> MTLKGMSYVMCTGSFKLEKE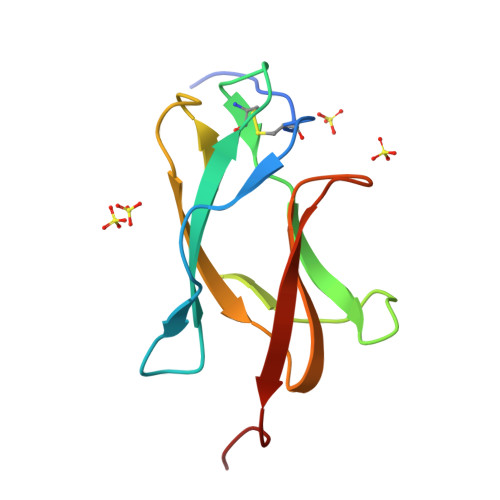VAETQHGTVLVQVKYEGTDAPCKIPFSTQDEKGATQNGRLITANPIVTDKEKPVNIEAEPPFGESYIVVGAGEKALKLSWFKKGSSIG>[2x]GPGHMVVKFSYMWTINNFSFCREEMGEVIKSSTFSSGANDKLKWCLRVNPKGLDEESKDYLSLYLLLVSCPKSEVRAKFKFSILNAKGEETKAMESQRAYRFVQGKDWG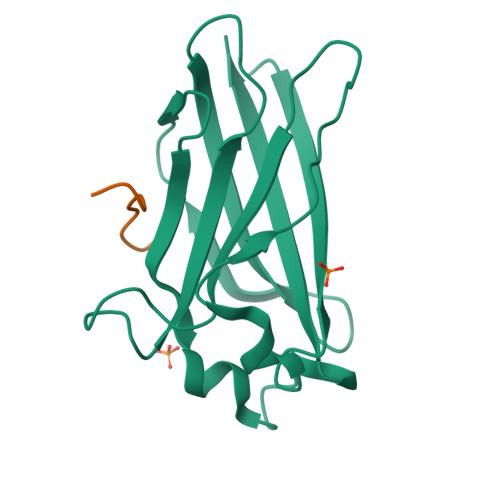FKKFIRRGFLLDEANGLLPDDKLTLFCEVSVVQD;>[2x]AEGTVSSSTDALPCI>GAMGPVDEQWIEILRIQALCARYCLTINTQDGEGWAGCFTEDGAFEFDGWVIRGRPALREYADAHARVVRGRHLTTDLLYEVDGDVATGRSASVVTLATAAGYKILGSGEYQDRLIKQDGQWRIAYRRLRN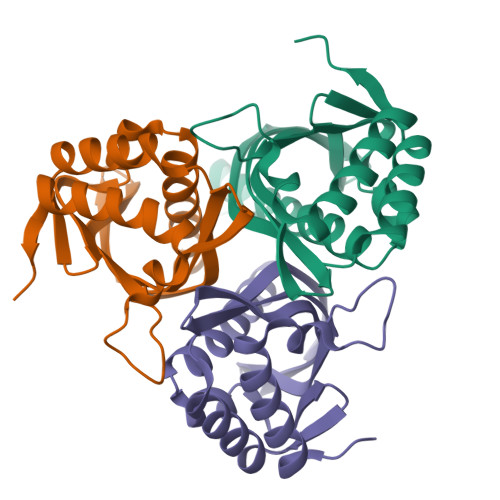DRLVSDPSVAVNVADADVAAVVGHLLAAARRLGTQMSDT[3x]methyl 4-azanyl-1-oxidanyl-2-oxidanylidene-1,8-naphthyridine-3-carboxylate | C10 H9 N3 O4 | 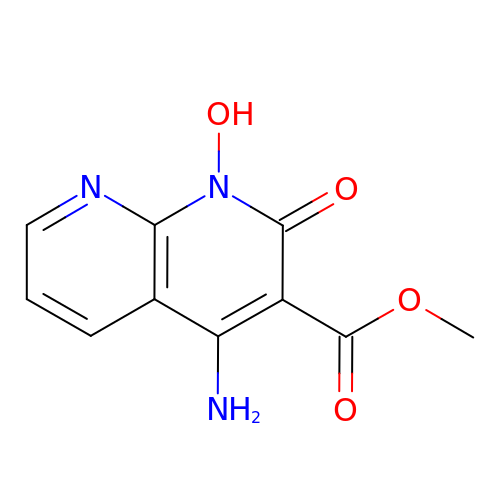DNQZHISFLXUWFF-UHFFFAOYSA-N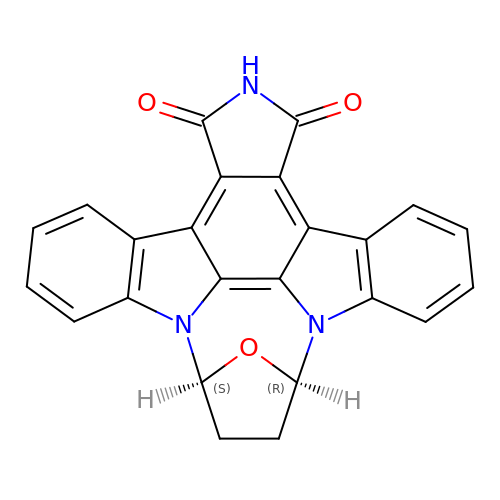REL-(9R,12S)-9,10,11,12-TETRAHYDRO-9,12-EPOXY-1H-DIINDOLO[1,2,3-FG:3',2',1'-KL]PYRROLO[3,4-I][1,6]BENZODIAZOCINE-1,3(2H)-DIONE | C24 H15 N3 O3 | OTPNDVKVEAIXTI-IYBDPMFKSA-N>ETGCKPEYSYAIAKNDRIGPLGAEGLTTVWKDYSPEMTLEDTMVIASCRDGKFMYLSRCTRETRYLAILHSRALPTSVVFKKLFEGQKQGDTVEMDDDFEFGLCPCDAKPIVRGKYNTTLLNGPAFQMVCPIGWTGTVSCMLANRDTLDTAVVRTYRRSRPFPYRQGCITQKVLGEDLYDCILGGNWTCVTGDQLQYSGGSIESCKWCGFKFQRSEGLPHYPIGKCRLKNETGYRLVDNTSCNREGVAIVPQGTVKCKIGDTTVQVIALDTKLGPM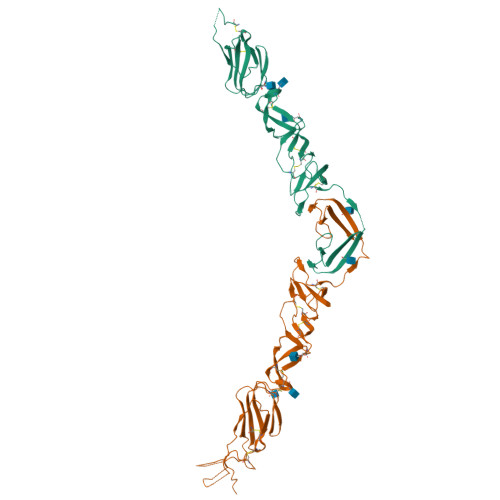PCKPYEIISSEGPVEKTACTFNYTKTLKNKYFEPRDSYFQQYMLKGEYQYWFDLEVTDGTK[2x]>[2x]UUCG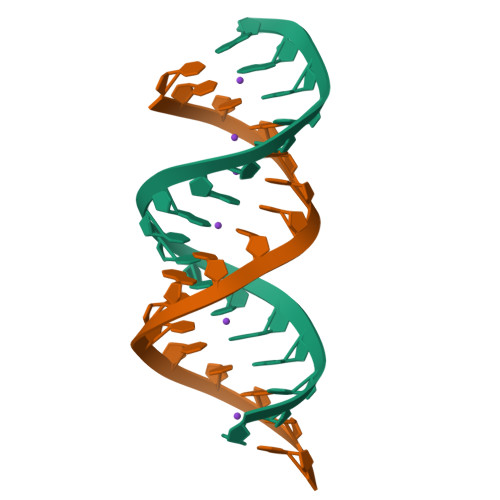GUUUUGAUCCGGA> MGSSHHHHHHSQDPMAIEADSVTRMNELLEILPAKQREILILR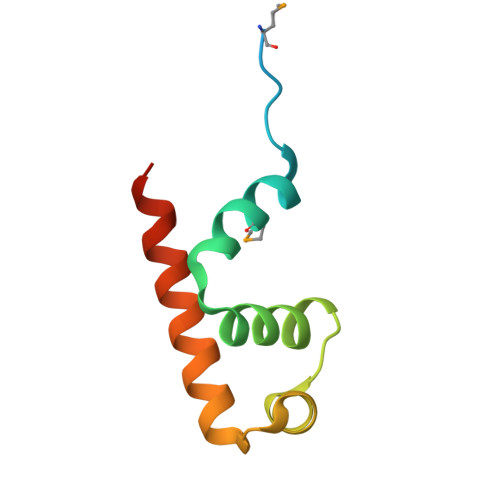VVVGLSAEETAAAVGSTTGAVRVAQHRALQRLKDEIVAAGDYA The PotD-PotABC protein complex in Escherichia coli, belonging to the adenosine triphosphate–binding cassette transporter family, is a spermidine-preferential uptake system. In general, ATP binding, hydrolysis, and phosphate release trigger conformational changes in the transporter, leading to the uptake of extracellular polyamines. Here, we report structural details of the polyamine uptake system PotD-PotABC in various states.

However, no ligand was observed in the structure; perhaps because of flexibility, this further corroborates the necessity of the E to Q mutation (E173Q).

>[2x]MGQSKKLNKQPSSLSPLVQLAGIRKCFDGKEVIPQLDLTINNGEFLTLLGPSGCGKTTVLRLIAGLETVDSGRIMLDNEDITHVPAENRYVNTVFQSYALFPHMTVFENVAFGLRMQKTPAAEITPRVMEALRMVQLETFAQRKPHQLSGGQQQRVAIARAVVNKPRLLLLDESLSALDYKLRKQMQNELKALQRKLGITFVFVTHDQEEALTMSDRIVVMRDGRIEQDGTPREIYEEPKNLFVAGFIGEINMFNATVIERLDEQRVRANVEGRECNIYVNFAVEPGQKLHVLLRPEDLRVEEINDDNHAEGLIGYVRERNYKGMTLESVVELENGKMVMVSEFFNEDDPDFDHSLDQKMAINWVESWEVVLADEEHK;> MKNTSKFQNVVIVTIVGWLVLFVFLPNLMIIGTSFLTRDDASFVKMVFTLDNYTRLLDPLYFEVLLHSLNMALIATLACLVLGYPFAWFLAKLPHKVRPLLLFLLIVPFWTNSLIRIYGLKIFLSTKGYLNEFLLWLGVIDTPIRIMFTPSAVIIGLVYILLPFMVMPLYSSIEKLDKPLLEAARDLGASKLQTFIRIIIPLTMPGIIAGCLLVMLPAMGLFYVSDLMGGAKNLLIGNVIKVQFLNIRDWPFGAATSITLTIVMGLMLLVYWRASRLLNKKVELE;> MIGRLLRGGFMTAIYAYLYIPIIILIVNSFNSSRFGINWQGFTTKWYSLLMNNDSLLQAAQHSLTMAVFSATFATLIGSLTAVALYRYRFRGKPFVSGMLFVVMMSPDIVMAISLLVLFMLLGIQLGFWSLLFSHITFCLPFVVVTVYSRLKGFDVRMLEAAKDLGASEFTILRKIILPLAMPAVAAGWVLSFTLSMDDVVVSSFVTGPSYEILPLKIYSMVKVGVSPEVNALATILLVLSLVMVIASQLIARDKTKGNTGDVK(1S)-1-[2-(difluoromethyl)pyridin-4-yl]-4-fluoro-1-(3-pyrimidin-5-ylphenyl)-1H-isoindol-3-amine 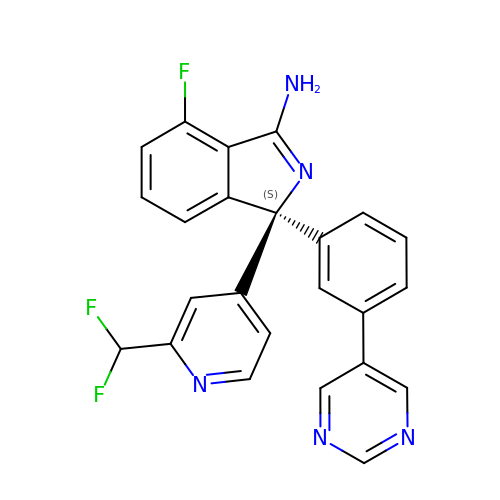| C24 H16 F3 N5 | MRXBCEQZNKUUIP-DEOSSOPVSA-N>[2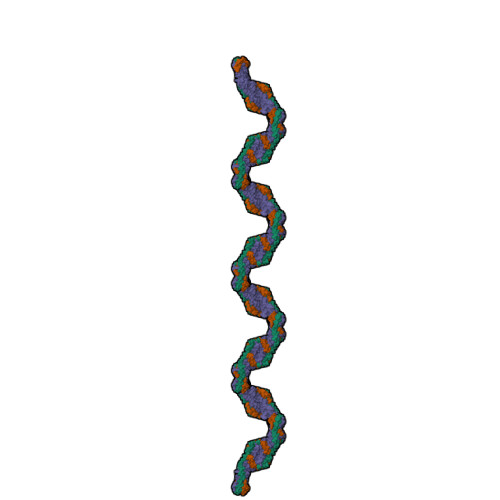x]MNHFGAVKSEEKYYIDADLLREIKQHLKQQQEGLSHLISIIKDDLEDIKLV;> GSHMAPADYFRVLVQQFEVQLQQYRQQIEELENHLATQANNSHITPQDLSMAMQKIYQTFVALAAQLQSIHENVKVLKEQYLSYRKMFLGDAG>[2x]PMI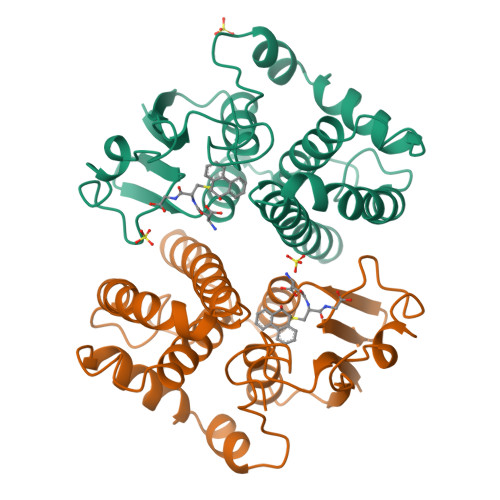LGFWNVRGLTHPIRLLLEYTDSSYEEKRYAMGDAPDYDRSQWLNEKFKLGLDFPNLPYLIDGSRKITQSNAIMRYLARKHHLCGETEEERIRADIVENQVMDNRMQLIMLCYNPDFEKQKPEFLKTIPEKMKLYSEFLGKRPWFAGDKVTYVDFLAYDILDQYHIFEPKCLDAFPNLKDFLARFEGLKKISAYMKSSRYLSTPIFSKLAQWSNK hMPV F is a class I fusion glycoprotein, synthesized as an inactive precursor (F0) that needs to be cleaved to become fusion competent. Proteolytic cleavage generates two disulfide-linked subunits (F2 N-terminal to F1) that assemble into a homotrimer. Finally, the fusion (F) glycoprotein mediates fusion of the viral and cellular membranes to allow entry of the viral ribonucleoprotein into the cell cytoplasm and thus initiate a new infectious cycle. To initiate membrane fusion, hMPV F is activated by still ill-defined mechanisms leading to a series of stepwise conformational changes in the F protein that drive membrane fusion and result in hMPV F adopting a highly stable “postfusion” conformation.

In order to advance our understanding of hMPV F structure and antigenicity (which lags behind other paramyxoviruses), we engineered a homogeneous preparation of soluble hMPV F folded in its postfusion conformation. This process required genetic manipulations that were not necessary for other paramyxovirus F proteins. We also crystallized the stabilized hMPV F postfusion trimer and determined its structure by X-ray diffraction analysis. Refolding of this intermediate leads to merging of the viral and target membranes concurrently with the assembly of HRA and HRB sequences of the F1 subunit into a highly stable six-helix bundle (6HB), which is characteristic of the postfusion conformation. Indeed, we found that 101F binds to hMPV F and cross-neutralizes hMPV. The structure is similar to that of the related human respiratory syncytial virus (hRSV) F glycoprotein, and two neutralizing epitopes are particularly well conserved, thus providing a structural basis for the cross-neutralizing activity of several monoclonal antibodies. Although immunization of BALB/c mice with purified postfusion hMPV F induced very limited cross-binding and cross-neutralization with hRSV, the elicited sera had robust neutralizing activity against hMPV, indicating that the hMPV postfusion F protein may be an effective subunit vaccine antigen.

>[6x]LKESYLEESCSTITEGYLSVLRTGWYTNVFTLEVGDVENLTCADGPSLIKTELDLTKSALRELRTVSADQLAREEQIENPRQSKKRKRR;>VATAAAVTAGVAIAKTIRLESEVTAIKNALKKTNEAVSTLGNGVRVLATAVRELKDFVSKNLTRAINKNKCDIADLKMAVSFSQFNRRFLNVVRQFSDNAGITPAISLDLMTDAELARAVSNMPTSAGQIKLMLENRAMVRRKGFGILIGVYGSSVIYMVQLPIFGVIDTPCWIVKAAPSCSEKKGNYACLLREDQGWYCQNAGSTVYYPNEKDCETRGDHVFCDTAAGINVAEQSKECNINISTTNYPCKVSTGRHPISMVALSPLGALVACYKGVSCSIGSNRVGIIKQLNKGCSYITNQDADTVTIDNTVYQLSKVEGEQHVIKGRPVSSSFDPVKFPEDQFNVALDQVFESIENSQALVDQSNRILSSAEKGNTSGRENLYFQ[6x]2-fluorobenzoic acid | C7 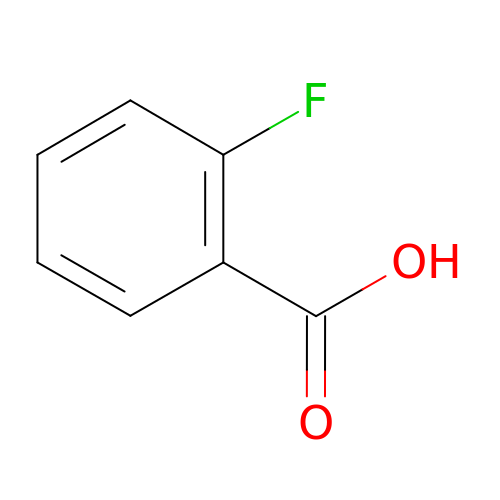H5 F O2 | NSTREUWFTAOOKS-UHFFFAOYSA-N> MAGKAHRLSAEERDQLLPNLRAVGWNELEGRDAIFKQFHFKDFNRAFGFMTRVALQAEKLDHHPEWFNVYNKVHITLSTHECAGLSERDINLASFIEQVAVSM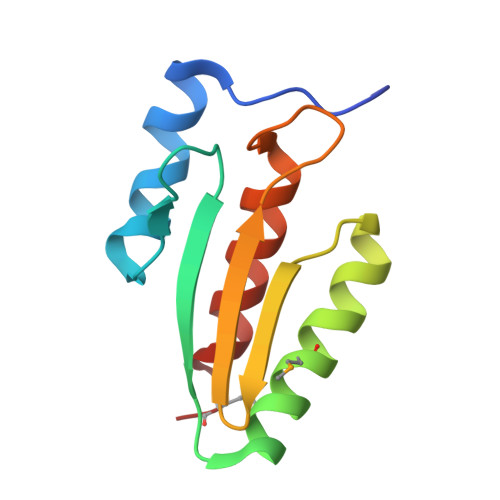T> MNDAAEVALYERLLQLRVLPGASDVHDVRFVFGDDSRCWIEVA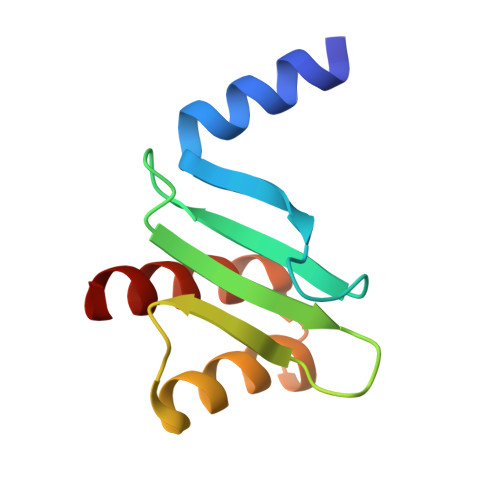MHGDHVIGNSHPALDPKSRATLEHVLTVQGDLAAFLVVARDMLLASL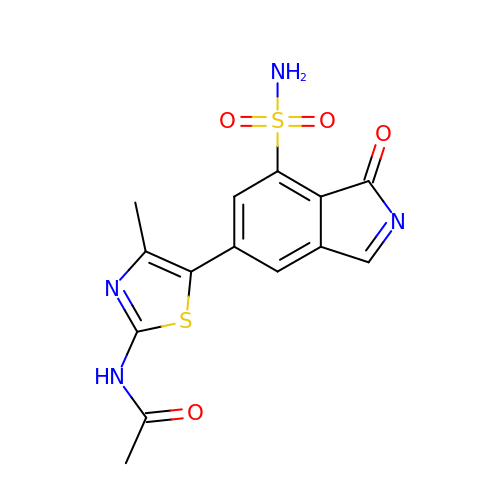~{N}-[4-methyl-5-(1-oxidanylidene-7-sulfamoyl-isoindol-5-yl)-1,3-thiazol-2-yl]ethanamide | C14 H12 N4 O4 S2 | LTKQWKJDTSYBED-UHFFFAOYSA-N>[4x]MAHHHHHHSTAIVTNVKHYGG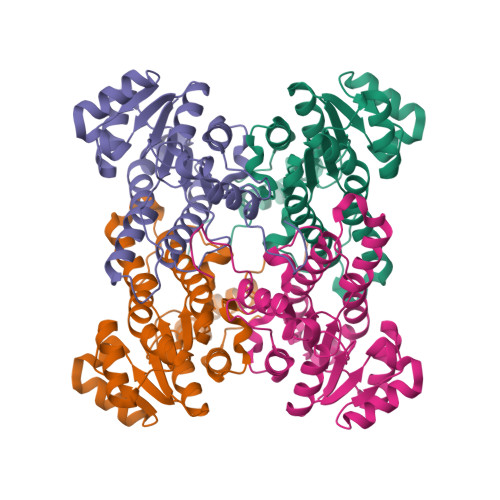MGSALRLSEAGHTVACHDESFKQKDELEAFAETYPQLKPMSEQEPAELIEAVTSAYGQVDVLVSNDIFATEWQPIDKYAVEDYRGAVEALQIRPFALVNAVASQMKKRKSGHIIFITSATPFGPWKELSTYTSARAGACTLANALSKELGEYNIPVFAIGPNYLHSEDSPYFYPTEPWKTNPEHVAHVKKVTALQRLGTQKELGELVAFLASGSCDYLTGQVFWLAGGFPMIERWPGMPE> XIMPPEAEIVPLPKLPMGALVPTAYGYIISDVPGETISAAISVAIPKDKSL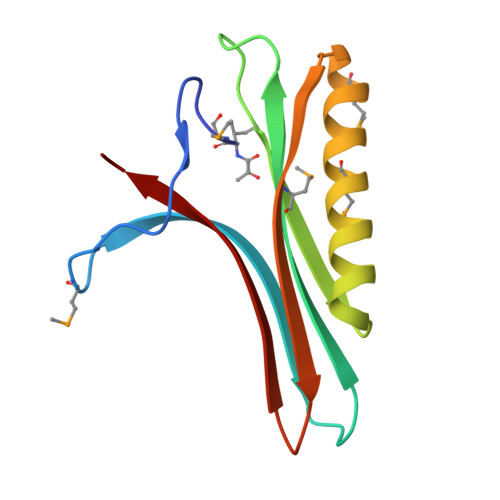CGLIMEYEGKCSKKEAEKTVREMAKIGFEMRGWELDRIESIAVEHTVEKLGCAFAAAALWYK>SNAMIVADSECRAELKDYLRFAPGGVGDSGPGEEQRESRARRGPRGPSAFIPVEEVLREGAESLEQHLGLEALMSSGRVDNLAVVMGLHPDYFTSFWRLHYLLLHTDGPLASSWRHYIAIMAAARHQCSYLVGSHMAEFLQTGGDPEWLLGLHRAPEKLRKLSEINKLLAHRPWLITKEHIQALLKTGEHTWSLAELIQALVLLTHCHSLSSFVFGCGILPEGDADGSPAPQAPTPPSEQSSPPSRDPLNNSGGFESARDVEALMERMQQLQESLLRDEGTSQEEMESRFELEKSESLLVTPSADILEPSPHPDMLCFVEDPTFGYEDFTRRGAQAPPT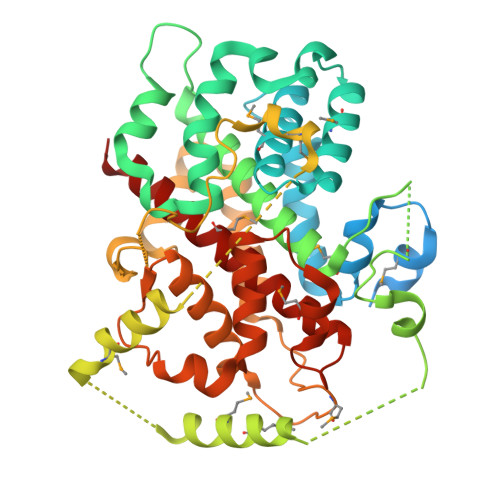FRAQDYTWEDHGYSLIQRLYPEGGQLLDEKFQAAYSLTYNTIAMHSGVDTSVLRRAIWNYIHCVFGIRYDDYDYGEVNQLLERNLKVYIKTVACYPEKTTRRMYNLFWRHFRHSEKVHVNLLLLEARMQAALLYALRAITRYMT[5x]>GEFTQSVSRLQSIVAGLKNAPSDQLINIFESCVRNPVENIMKILKGIGETFCQHYTQSTDEQPGSHIDFAVNRLKLAEILYYKILETVMVQETRRLHGMDMSVLLEQDIFHRSLMACCLEIVLFAYSSPRTFPWIIEVLNLQPFYFYKVIEVVIRSEEGLSRDMVKHLNSIEEQILESLAWSHDSALWEALQVSANKVPTCEEVIFPNNFETGNNRPKRTGSLALFYRKVYHLASVRLRDLCLKLDVSNELRRKIWTCFEFTLVHCPDLMKDRHLDQLLLCAFYIMAKVTKEERTFQEIMKSYRNQPQANSHVYRSVLLKSIKEERGDLIKF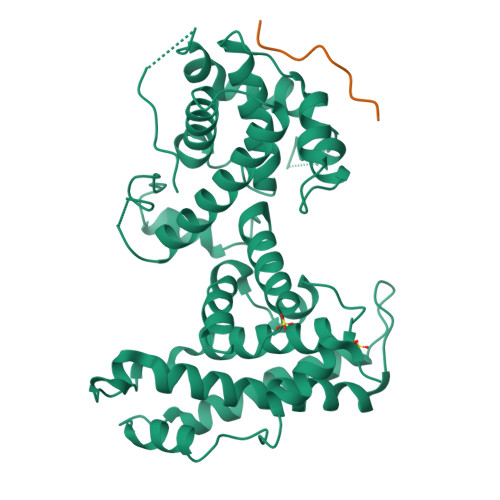YNTIYVGRVKSFALKYDLANQDHMMDAPPLSPFPHIKQQ[2x];>[2x]DIYCYEEFSD>[2x]MSVNGNLRSLIDMLEAAQDGHMIKIALRSFAHSCGYDRFAYLQKDGTQVRTFHSYPGPWESIYLGSDYFNIDPVLAEAKRRRDVFFWTADAWPARGSSPLRRFRDEAISHGIRCGVTIPVEGSYGSAMMLTFASPERKVDISGVLDPKKAVQLLMMVHYQLKIIAAKTVLNPKQMLSPREMLCLVWASKGKTASVTANLTGINARTVQHYLDKARAK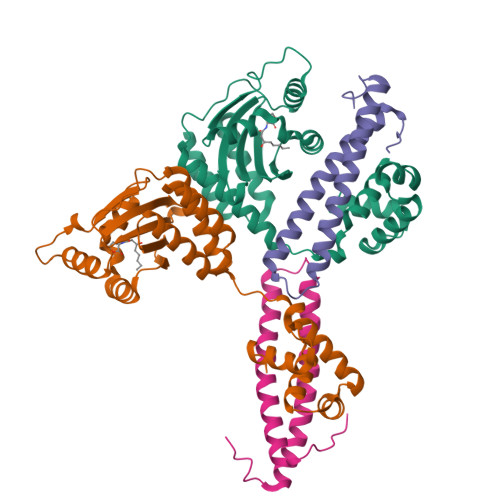LDAESVPQLVAIAKDRGLV;>MNDMGSSEVNDENKEKEARYSVMTKSELEALAVSAIREHRRLLWADQAVYEEWLRASDDPSISGPVLQTLQDEYVARQKRSEAQQEELSDILDALGFVPDVPFDDDN[2x]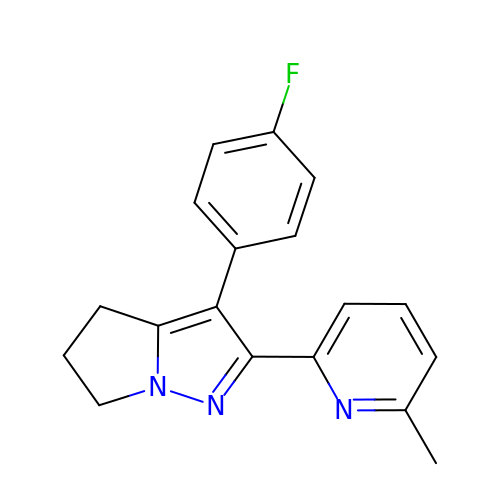3-(4-FLUOROPHENYL)-2-(6-METHYLPYRIDIN-2-YL)-5,6-DIHYDRO-4H-PYRROLO[1,2-B]PYRAZOLE | C18 H16 F N3 | NBDZLUOYAAVYHF-UHFFFAOYSA-N>MAKPANKLVIVTEKILLKKIAKIIDESGAKGYTVMNTGGKGSRNVRSSGQPNTSDIEANIKFEILTETREMAEEIA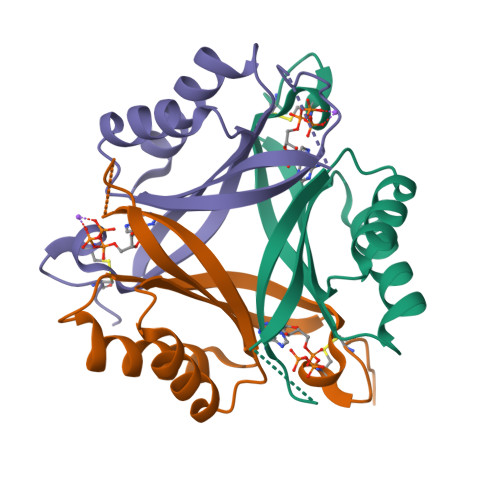DRVAVKYFNDYAGIIYICSAEVLYGHTFCGPEGCSAWSHPQFEK[3x]>[2x]MGHHHHHHHHHHSSGHIEGRHMAAHQLSDFQRNKILRVFNTFYDCNHD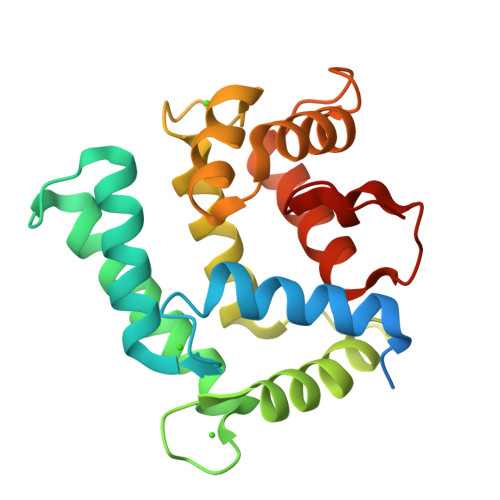GVIEWDDFELAIKKICNLHSWPTDGKKHNEARADLKLIWDGLRKYADENEDEQVTKEEWLKMWAECVKSVEKGESLPEWLTKYMNFMFDVNDTSGDNIIDKHEYSTVYMSYGIPKSDCDAAFDTLSDGGKTMVTREIFARLWTEYFVSNDRGAKGNHLFGDLKL>[3x]MGDTKEQRILRYVQQHAKPGDPQSVLEAIDTYCTQKEWAMNVGDAKGQIMDEVIQEHNPSLVLELGAYCGYSAVRMARLLSPGARLLTMEKNPDY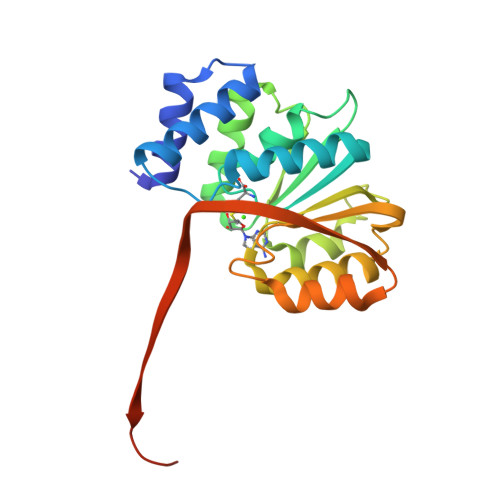AAITQQMLNFAGLQDKVTILIGASQDLIPQLKKYDVDTLDLVFLDHWKDRYLPDTILLEECGLLRKGTVLLADNVIVPGTPDFLAYVRGSSSFECTHYSSYLEYMKVVDGLEKAVYKGPSSPKQPLEHHHHHH>[4x]MISETIRSGDWKGEKHVPVIEYEREGELV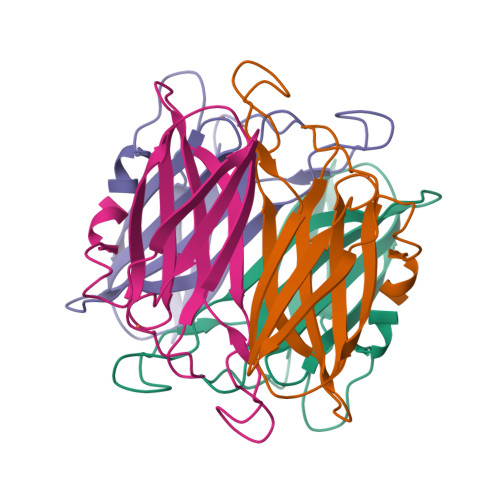KVKVQVGKEIPHPNTTEHHIRYIELYFLPEGENFVYQVGRVEFTAHGESVNGPNTSDVYTEPIAYFVLKTKKKGKLYALSYCNIHGLWENEVTLE> GKAFDDGAFTGIREINLSYNKETAIGDFQVVYDLNGSPYVGQNHVSFITG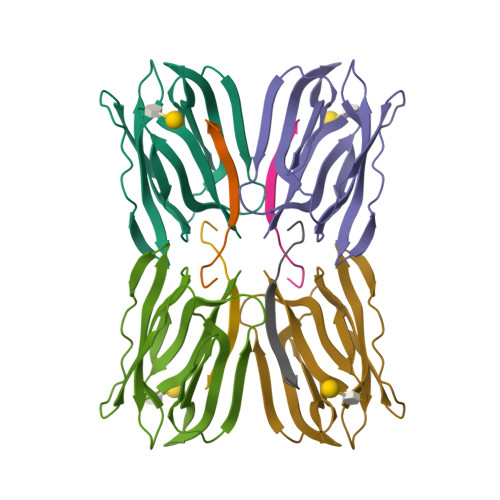FTPVKISLDFPSEYIMEVSGYTGNVSGYVVVRSLTFKTNKKTYGPYGVTSGTPFNLPIENGLIVGFKGSIGYWLDYFSMYLSL;> DEQSGISQTVIVGPWGAKVS>GGGGGGHMKIIIAGKNDIAVNVTRWLQKKKKNIEIYAICNANDTGIDTFQRSFKKYCKDNLIPIISLAEAYKIDDAIFLSLEFDKIVQPSKFNHNELFNIHFSYLPKYKGMYTSAWPILNGEDTSGVTLHKIDHGIDTGAIIAQKEIIIQPFETAKDLYEKYISEGTSLVIDNISTLLNSEYVEKEQNIKYSSYYSKKTIDYSNLELNFSKTAFEIINQLRAFTFREYQLPKLDGVNIFLGDVLSSRSIMKPGSILERNDKEIIVSTIDYDVVLYKDNFKEILEACKYSDSKYIAKLIRAKSILFEKNIYGWSPVIVAAYHGNIELIKWLVSKGANINDRNYKGTTVAMYFKDYMLK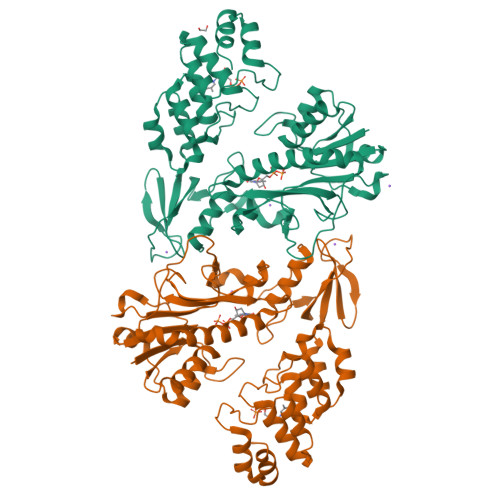SGDYSGLKMLIDLGLDLTLTDYKDYTVFDYLEKSGNKNLLQYMMAFMK[2x]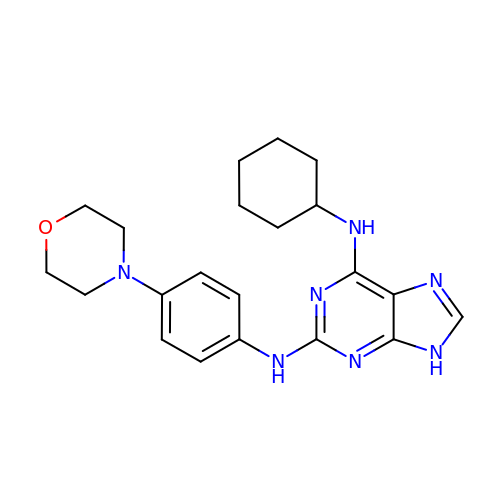N~6~-cyclohexyl-N~2~-(4-morpholin-4-ylphenyl)-9H-purine-2,6-diamine | C21 H27 N7 O | ZFLJHSQHILSNCM-UHFFFAOYSA-N(4Z,7Z,10Z,13Z,16R,17R,19Z)-16,17-dihydroxydocosa-4,7,10,13,19-pentaenoic 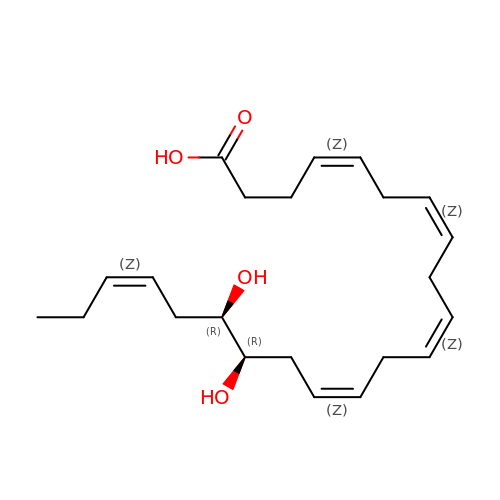acid | C22 H34 O4 | YXQCSWUATWXVGK-QJJBBLQJSA-N> GASYFTSVDQSSVHTAEVGSHQIEPLKTSVDKPGSKKTQGEKFFLIHSARWLTTHALFHEVAKLDVVKLLYNEQFAVQGLLRYHTYARFGIEIQVQINPTPFQQGGLICAMVPGDQSYGSIASLTVYPHGLLNCNIN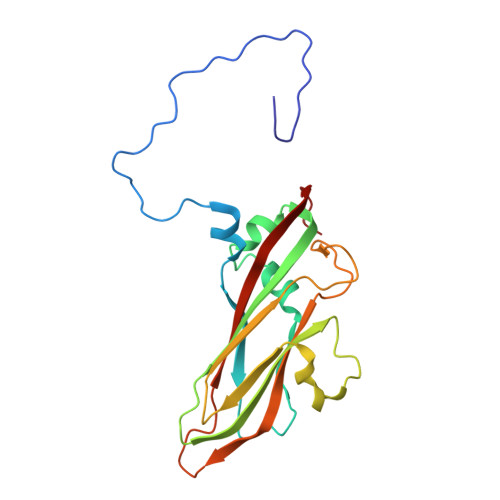NVVRIKVPFIYTRGAYHFKDPQYPVWELTIRVWSELNIGTGTSAYTSLNVLARFTDLELHGLTPLST D-rhamnopyranose tetrazole | C6 H10 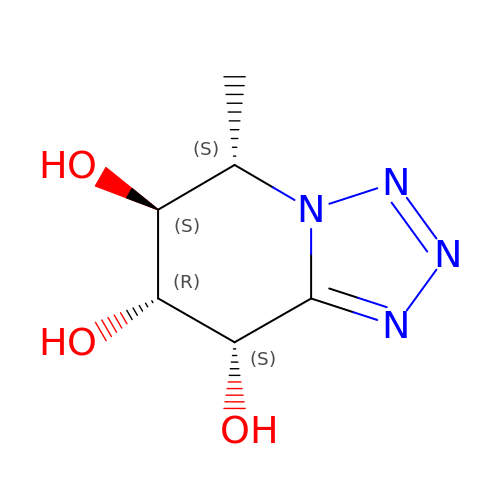N4 O3 | RGTARVZVTUMUSY-QMKXCQHVSA-N> GITALRQQVETLQGQVQRLQKAFSQYKKVELFPNGRGVGEKI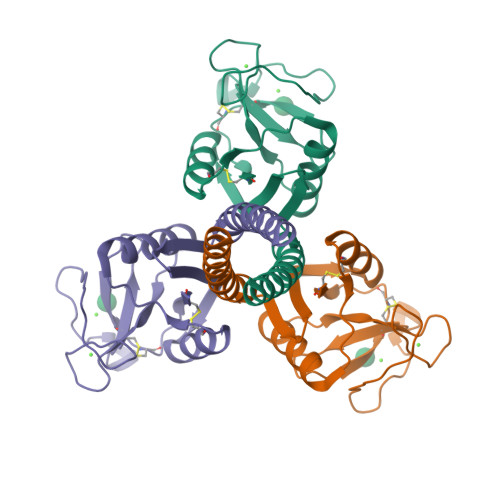FKTGGFEKTFQDAQQVCTQAGGQMASPRSETENEALSQLVTAQNKAAFLSMTDIKTEGQFTYPTGEPLVYANWAPGEPNNNGGSSGAENCVEIFPNGKWNDKACGELRLVICEF> VKELLEAGVHFGHERKRWNPKFARYIYAERNGIHIIDLQKTMEELERTFRFIEDLAMRGGTILFVGTKKQAQDIVRMEAERAGMPYVNQRWLGGMLTNFKTIQRVHRLEELEALFASPEIEERPKKEQRLHELERLQKYLSGFRLLKRLPDAIFVVDPTKEAIAVREARKLFIPVIALADTDSDPDLVDYIIPGNDDAIRSIQLILSRAVDLIIQARGGVVEPSPSYALVQ;> ARRRRAEVRQLQPDLVYGDVLVTAFINKIMRDGKKNLAARIFYDACKIIQEKTGQEPLKVFKQAVENVKPRMEVRSRRVGGANYQVPMEVSRRQQSLALRWLVQAANQRPERRAAVRIAHELMDAAEGKGGAVKKKEDVERMAEANRAYAHYRW;> KRQVASGRAYIHASYNNTIVTITDPDGNPITWSSGGVIGYKGSRKGTPYAAQLAALDAAKKAMAYGMQSVDVIVRGTGAGREQAIRALQASGLQVKSIVDDTPVPHNGCRPKKKFRKAS;> PSRKAKVKATLGEFDLRDYRNVEVLKRFLSETGKILPRRRTGLSGKEQRILAKTIKRARILGLLPFTEKLVRK;> DKSYCGFIAIVGRPNVGKSTLLNKLLGQKISITSRKAQTTRHRIVGIHTEGAYQAIYVDTPGLHMEEKRAINRLMNKAASSSIGDVELVIFVVEGTRWTPDDEMVLNKLREGKAPVILAVNKVDNVQEKADLLPHLQFLASQMNFLDIVPISAETGLNVDTIAAIVRKHLPEATHHFPE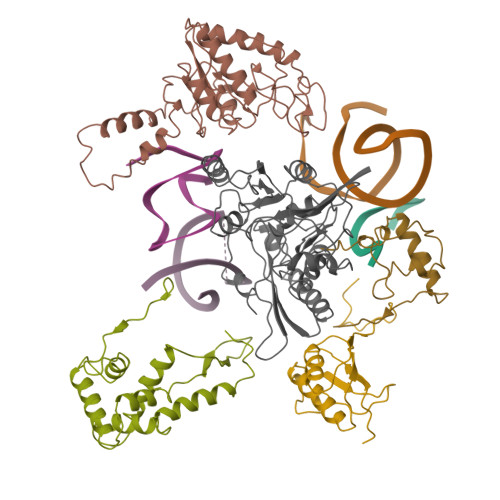DYITDRSQRFMASEIIREKLMRFLGAELPYSVTVEIERFVSNERGGYDINGLILVEREGQKKMVIGNKGAKIKTIGIEARKDMQEMFEAPVHLELWVKVKSGWADDERALRSL> SWK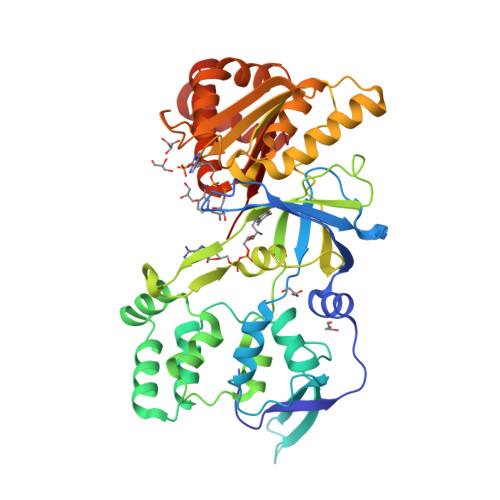RNKFRLTYVAEAPDLTQGLSNVHKKRVSAARLLSRQNLQSPKSSRSTIFVRLHTNGNQELQYQPGDHLGVFPGNHEDLVNALIERLEDAPPANHVVKVEMLEERNTALGVISNWKDESRLPPCTIFQAFKYYLDITTPPTPLQLQQFASLATNEKEKQRLLVLSKGLQEYEEWKWGKNPTMVEVLEEFPSIQMPATLLLTQLSLLQPRYYSISSSPDMYPDEVHLTVAIVSYHTRDGEGPVHHGVCSSWLNRIQADDVVPCFVRGAPSFHLPRNPQVPCILVGPGTGIAPFRSFWQQRQFDIQHKGMNPCPMVLVFGCRQSKIDHIYREETLQAKNKGVFRELYTAYSREPDRPKKYVQDVLQEQLAESVYRALKEQGGHIYVCGDVTMAADVLKAIQRIMTQQGKLSEEDAGVFISRLRDDNRYHEDIFGV>[6x]KSSHTLKTANSYTDVTVSNSTKKAIRESNQYTDHKMHQLENRLDKLEKR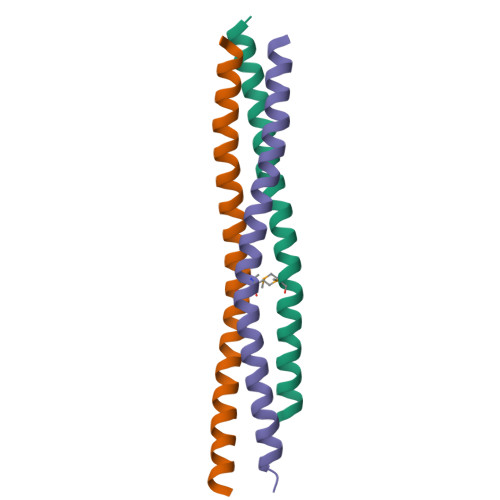LLKLLASSAALNSLF> CGCGAAUUAGCG

We have developed the hydrazine/NH4Cl/OsO4‐based conversion of 6‐thioguanosine (6sG) into A′, where A′ constitutes a 6‐hydrazino purine derivative. A′ retains the Watson–Crick base‐pair mode and is efficiently decoded as adenosine in primer extension assays and in RNA sequencing. Because 6sG is applicable to metabolic labeling of freshly synthesized RNA and because the conversion chemistry is fully compatible with the conversion of the frequently used metabolic label 4‐thiouridine (4sU) into C, the combination of both modified nucleosides in dual‐labeling setups enables high accuracy measurements of RNA decay. This approach, termed TUC‐seq DUAL, uses the two modified nucleosides in subsequent pulses and their simultaneous detection, enabling mRNA‐lifetime evaluation with unprecedented precision.

Encouraged by these findings, we thoroughly characterized the novel A′ modification. As expected, the thermodynamic stability of an A′–U base pair was comparable to native A–U base pairs in short RNA oligonucleotides. Furthermore, when we crystallized a short palindromic RNA duplex containing the A′ modification and solved its crystal structure at 1.0 Å resolution, we found that the Watson–Crick mode for A′ pairing with U and the double helical geometry were retained, as encountered in the native duplex. Next, we tested the impact of the modifications on reverse transcription in a primer extension assay using Superscript III reverse transcriptase. Likewise, the vast majority of A′‐containing RNA was reverse transcribed to the full‐length product and only a slight increase in termination was observed. As expected, A′ was read as A (see ddTTP sequencing lane).>[3x]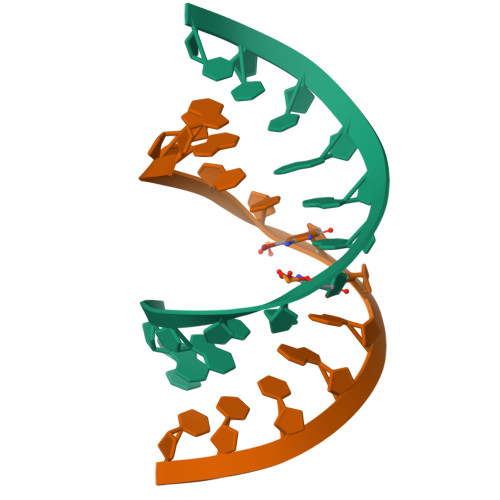GGACUCGAAUCC> MSNKEKNASETRKAYTTKMIPRSHDRMKLLGNFMDYLMDGTPIFFELWNQFGGGIDRDIISGTANKDKISDDLLLAVNWFKVMPINSKPQGVSPSNLANLFQQYSGSEPDIQAQEYFASNFDTEKHQWKDMRVEYERLLAELQLSRSDMHHDLKLMYKEKCIGLSLSTAHYITSVMFGTGAKNNRQTKHQFYSKVIQLLEESTQINSVEQLASIILKAGDCDSYRKLRIRCSRKGATPSILKIVQDYELGTNHDDEVNVPSLIANLKEKLGRFEYECEWKCMEKIKAFLASKVGPYYLGSYSAMLENALSPIKGMTTKNCKFVLKQIDAKNDIKYENEPFGKIVEGFFDSPYFESDTNVKWVLHPHHIGESNIKTLWEDLNAIHSKYEEDIASLSEDKKEKRIKVYQGDVCQTINTYCEEVGKEAKTPLVQLLRYLYSRKDDIAVDKIIDGITFLSKKHKVEKQKINPVIQKYPSFNFGNNSKLLGKIISPKDKLKHNLKCNRNQVDNYIWIEIKVLNTKTMRWEKHHYALSSTRFLEEVYYPATSENPPDALAARFRTKTNGYEGKPALSAEQIEQIRSAPVGLRKVKKRQMRLEAARQQNLLPRYTWGKDFNINICKRGNNFEVTLATKVKKKKEKNYKVVLGYDANIVRKNTYAAIEAHANGDGVIDYNDLPVKPIESGFVTVESQVRDKSYDQLSYNGVKLLYCKPHVESRRSFLEKYNGTMKDNRGNNIQIDFMKDFEAIADDETSLYYFNMKYCKLLQSSIRNHSSQAKEYREEIFELLRDGKLSVLKLSSLSNLSFVMFKVAKSLIGTYFGHLLKKPKNSKSDVKAPPITDEDKQKADPEMFALRLALEEKRLNKVKSKKEVIANKIVAKALELRDKYGPVLIKGENISDTTKKGKK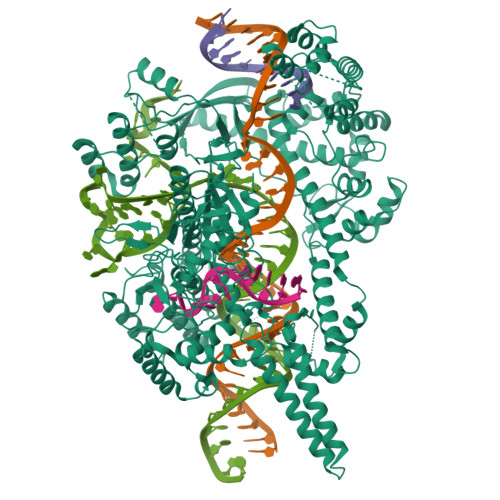SSTNSFLMDWLARGVANKVKEMVMMHQGLEFVEVNPNFTSHQDPFVHKNPENTFRARYSRCTPSELTEKNRKEILSFLSDKPSKRPTNAYYNEGAMAFLATYGLKKNDVLGVSLEKFKQIMANILHQRSEDQLLFPSRGGMFYLATYKLDADATSVNWNGKQFWVCNADLVAAYNVGLVDIQKDFKKK> MVDAEMAAFGEAAPYLRKSEKERLEAQTRPFDLKKDVFVPDDKEEFVKATILSREGGKVTAETEHGKTVTVKEDQVLQQNPPKFDKIEDMAMLTFLHEPAVLYNLKERYASWMIYTYSGLFCVTINPYKWLPVYNAEVVAAYRGKKRSEAPPHIFSISDNAYQYMLTDRENQSILITGESGAGKTVNTKRVIQYFAVIAAIGDRSKKEQATGKGTLEDQIIQANPALEAFGNAKTVRNDNSSRFGKFIRIHFGATGKLASADIETYLLEKSRVIFQLKAERDYHIFYQILSNKKPELLDMLLITNNPYDYAFISQGETTVASIDDAEELMATDNAFDVLGFTTEEKNSMYKLTGAIMHFGNMKFKLKQREEQAEPDGTEEADKSAYLMGLNSADLLKGLCHPRVKVGNEYVTKGQNVQQVVYAKGALAKAVYERMFNWMVTRINATLETKQPRQYFIGVLDIAGFEIFDFNSFEQLCINFTNEKLQQFFNHHMFVLEQEEYKKEGIEWEFIDFGMDLQACIDLIEKPMGIMSILEEECMFPKATDMTFKAKLFDNHLGKSSNFQKPRNIKGKPEAHFSLIHYAGTVDYNIIGWLQKNKDPLNETVVDLYKKSSLKMLSSLFANYAGFDTPIEKGKGKAKKGSSFQTVSALHRENLNKLMTNLRSTHPHFVRCIIPNETKSPGVIDNPLVMHQLRCNGVLEGIRICRKGFPNRILYGDFRQRYRILNPAAIPEGQFIDSRKGAEKLLGSLDIDHNQYKFGHTKVFFKAGLLGLLEEMRDERLSRIITRIQAQSRGVLSRMEFKKLLERRDSLLIIQWNIRAFMGVKNWP

In cardiac muscle, cardiac myosin comprises, in part, the thick filament of the cardiac sarcomere and powers cardiac contractility. The force produced by myosin motors is generated by coupling the sequential release of the products of ATP hydrolysis (Phosphate (Pi) and ADP) to a series of strong actin-binding states and the swing of a distal elongated domain of myosin called the lever arm. Omecamtiv mecarbil (OM) is a selective, small-molecule cardiac myosin activator that binds to the catalytic domain of myosin and increases cardiac contractility in preclinical models without affecting cardiac myocyte intracellular calcium concentrations or myocardial oxygen consumption. Here, we describe a previously unseen conformation of the bovine cardiac myosin motor in the PPS state that OM stabilizes and binds to with high affinity.

Comparison of the structures with and without drug bound reveals that the OM-binding pocket is actually not completely formed in the APO-MD-PPS structure. Interestingly, in the presence of OM, the lever arm adopts a primed lever arm position that is close to that previously observed for scallop myosin II, while the cardiac apo PPS structure has a lever arm position slightly less primed, with concerted changes in the relay and the converter position. Comparison of these two cardiac PPS structures reveals that drug binding does not significantly alter the structure of the motor domain. The two motor domains of OM-S1-PPS and APO-MD-PPS structures can be superimposed overall with a root-mean-square deviation (r.m.s.d.) of 0.88 Å for 557 Cα atoms between the OM bound and APO structures and with a r.m.s.d. of 1.33 Å for 593 Cα atoms if the relay and converter are also taken into consideration. Comparison with other myosin II isoforms in the same structural state reveals that the cardiac myosin PPS state is also very similar to that of Argopecten (scallop)-striated muscle myosin II (1QVI13, r.m.s.d. of 0.75 Å for 582 Cα atoms) and chicken smooth muscle myosin (SMM) II (1BR114, r.m.s.d. of 0.95 Å for 547 Cα atoms). Importantly, our structures indicate that OM does not change the conformations that the motor domain explores during the motor cycle but acts by increasing the stability of the states with lever arm primed.(3R)-4-({(2S)-1-[(5-acetamidopentyl)amino]-1-oxo-3-phenylpropan-2-yl}amino)-3-hydroxy-4-oxobutanoic acid | C20 H29 N3 O6 | 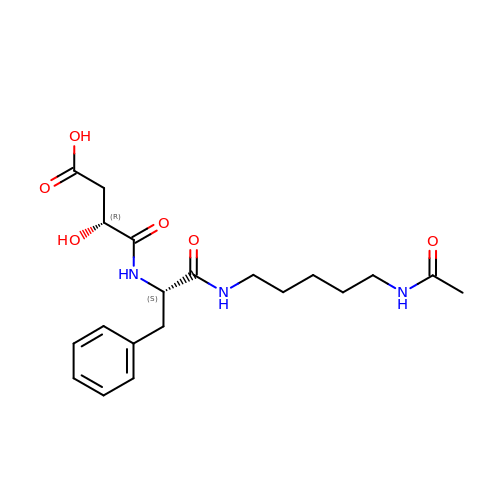DEIZDXKQOQMCEV-DLBZAZTESA-N> MATQEEILDAALVSGDSSQLTDSHLVALRLQQQVERIRQTRTQLLDGLYQNLSQAYDPGAASMWVLPANPDNTLPFLIGDKGRVLASLSLEAGGRGLAYGTNVLTQLSGTNAAHAPLLKRAVQWLVNGDPGAATAKDFKVSVVGVDKTAALNGLKSAGLQPADAACNALTDASCASTSKLLVLGNGASAASLSATVRARLQAGLPILFVHTNGWNQSSTGQQILAGLGLQEGPYGGNYWDKDRVPSSRTRTRSVELGGAYGQDPALVQQIVDGSWRTDYDWSKCTSYVGRTTCDDVPGLSDFSKRVDVLKGALDAYNQKAQNLFALPGTTSLRLWLLWADAVRQNIRYPMDKAADTARFQETFVADAIVGYVREAGAAQKELGSYAGQRQQSMPVSGSEETLTLTLPSAQGFTAIGRMAAPGKRLSIRIEDAGQASLAVGLNTQRIGSTRLWNTRQYDRPRFLKSPDIKLQANQSVALVSPYGGLLQLVYSGATPGQTVTVKVTGAASQPFLDIQPGEDSSQAIADFIQALDADKADWLEI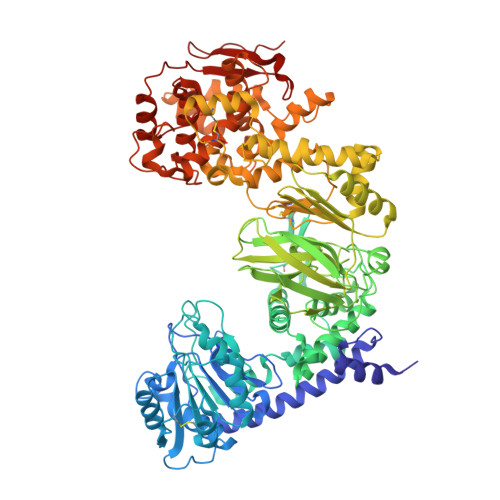RSGSVEVHAKVEKVRGSIDKDYGGDVQRFIRELNEVFIDDAYTLAGFAIPNQAKTPAIQQECAARGWDCDSETLHKLPGTQHINVDQYAQCGGGCSGNPYDQTWGLNPRGWGESHQLGHNLQVNRLKVYGGRSGEISNQIFPLHKDWRVLREFGQNLDDTRVNYRNAYNLIVAGRAEADPLAGVYKRLWEDPGTYALNGERMAFYTQWVHYWADLKNDPLQGWDIWTLLYLHQRQVDKSDWDANKAALGYGTYAQRPGNSGDASSTDGNDNLLLGLSWLTQRDQRPTFALWGIRTSAAAQAQVAAYGFAEQPAFFYANNRTNEYSTVKLLDMSQGSPAWPFPLE> MIQLKNVGITLSGKGYERFSLENINLEVNGEKVIILGPNGSGKTTLLRAISGLLPYSGNIFINGMEVRKIRNYIRYSTNLPEAYEIGVTVNDIVYLYEELKGLDRDLFLEMLKALKLGEEILRRKLYKLSAGQSVLVRTSLALASQPEIVGLDEPFENVDAARRHVISRYIKEYGKEGILVTHELDMLNLYKEYKAYFLVGNRLQGPISVSELLESSIVEGERNDALLVLDIMDKKVSIVKGDLGMKFG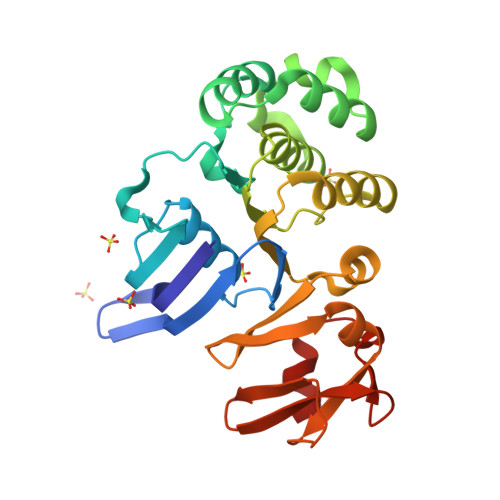ALGSLNRIYGIIGA>[2x]GAMAQNIT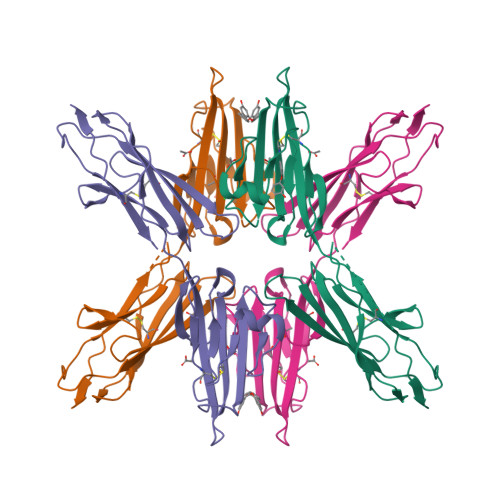ARIGEPLVLKCKGAPKKPPQRLEWKLNTGRTEAWKVLSPQGGGPWDSVARVLPNGSLFLPAVGIQDEGIFRCQAMNRNGKETKSNYRVRVYQIPGKPEIVDSASELTAGVPNKVGTCVSEGSYPAGTLSWHLDGKPLVPNEKGVSVKEQTRRHPETGLFTLQSELMVTPARGGDPRPTFSCSFSPGLPRHRALRTAPIQPRVWE>[2x]SLIQFETLIMKVVKKSGMFWYSAYGCYCGWGGHGRPQDATDRCCFVHDCC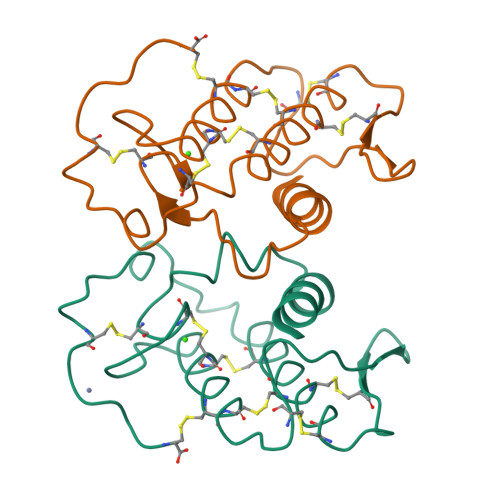YGKVTGCDPKMDSYTYSEENGDIVCGGDDPCKREICECDRVAADCFRDNLDTYNSDTYWRYPRQDCEESPEPC2-fluoranyl-5-[2-[(4~{S})-4-[4-methyl-1,1-bis(oxidanylidene)thian-4-yl]-2-oxidanylidene-pyrrolidin-1-yl]ethoxy]benzenecarbonitrile 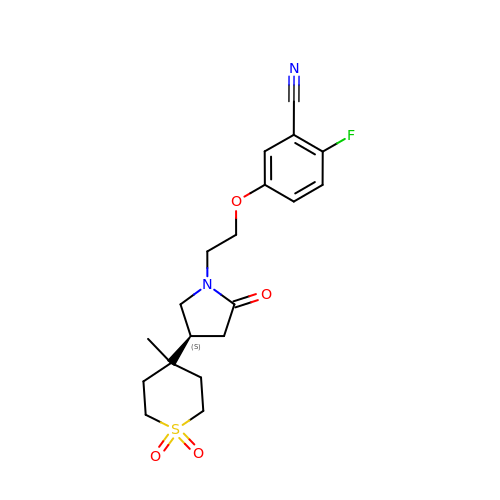| C19 H23 F N2 O4 S | SYEMWCXBADSSGE-OAHLLOKOSA-N>MGSHHHHHHDITSLYKKAGSENLYFQMKLRYLNILKEKLGREPTFVELQAFSVMWSEHCGYSHTKKYIRRLPKTGFEGNAGVVNLDDYYSVAFKIESHNHPSAIEPYNGAATGVGGIIRDVLAMGARPTAIFDSLHMSRIIDGIIEGIADYGNSIGVPTVGGELRISSLYAHNPLVNVLAAGVVRNDMLVDSKASRPGQVIVIFGGATGRDGIHGASFASEDLTGDKATKLSIQVGDPFAEKMLIEAFLEMVEEGLVEGAQDLGAGGVLSATSELVAKGNLGAIVHLDRVPLREPDMEPWEILISESQERMAVVTSPQKASRILEIARKHLLFGDVVAEVIEEPVYRVMYRNDLVMEVPVQLLANAPEEDIVEYTPGKIPEFKRVEFEEVNAREVFEQYDHMVGTDTVVPPGFGAAVMRIKRDGGYSLVTHSRADLALQDTYWGTLIAVLESVRKTLSVGAEPLAITNCVNYGDPDVDPVGLSAMMTALKNACEFSGVPVASGNASLYNTYQGKPIPPTLVVGMLGKVNPQKVAKPKPSKVFAVGWNDFELEREKELWRAIRKLSEEGAFILSSSQLLTRTHVETFREYGLKIEVKLPEVRPAHQMVLVFSERTPVVDVPVKEIGTLSR[3x];>MPLFKFAIDVQYRSNVRDPRGETIERVLREEKGLPVKKLRLGKSIHLEVEAENKEKAYEIVKKACEELLVNPVVEEYEVREL[6x];>MKPRACVVVYPGSNCDRDAYHALEINGFEPSYVGLDDKLDDYELIILPGGFSYGDYLRPGAVAAREKIAFEIAKAAERGKLIMGICNGFQILIEMGLLKGALLQNSSGKFICKWVD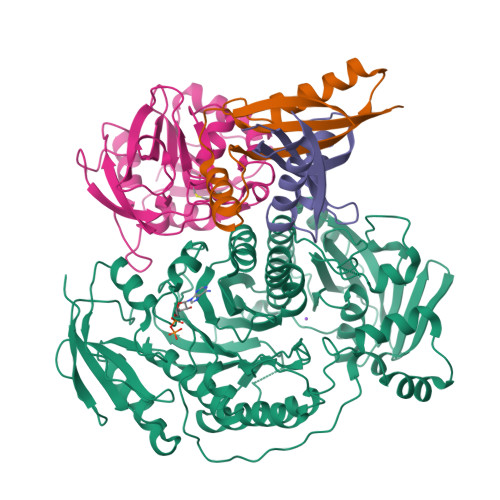LIVENNDTPFTNAFEKGEKIRIPIAHGFGRYVKIDDVNVVLRYVKDVNGSDERIAGVLNESGNVFGLMPHPERAVEELIGGEDGKKVFQSILNYLKR[3x]> MERLVWDKLTLLGFLEKNHIPQKLYYNLSSQDKELSAEIQSNVTYYTLRDANNTLIQALIPISQDLQIHIYKKGEDYFLDFIPIIFTRKEKTLLLSLQTSPYQDIIKATNDPLLANQLMNAYKKSVPFKRLVKNDKIAIVYTRDYRVGQAFGQPTIKMAMVSSRSNQYYLFSHSNGHYYDSKAQEVAGFLLETPVKYTRISSPFSYGRFHPVLKVRRPHYGVDYAAKHGSLIHSASDGRVGFMGVKAGYGKVVEIHLNELRLVYAHMSAFANGLKKGSFVKKGQIIGRVGSTGLSTGPHLHFGVYKNSRPINPLGYIRTAKSKLHGKQREVFLEKAQRSKQKLEELLKTHSFEKNSFYLLEGFLEHHHHHH

Seven cell shape-determining genes (csd1, csd2, csd3/hdpA, ccmA, csd4, csd5 and csd6) have been identified in H. pylori. Among them, Csd3 (also known as HdpA) is a bifunctional enzyme. Its d,d-endopeptidase activity cleaves the d-Ala4-mDAP3 peptide bond between cross-linked muramyl tetrapeptides and pentapeptides.

Among these, only the N-terminally 41-residue truncated Csd3 (Csd3Δ41) comprised of residues 42–403 was expressed in soluble form, and it yielded two different forms (the orthorhombic form 1 and the hexagonal form 2) of well diffracting crystals. We have determined the structure of Csd3Δ41 using SAD data from a Pt-derivatized form 2 crystal. The form 2 crystal contains one monomer of Csd3Δ41 in the asymmetric unit. This model of Csd3Δ41 excludes six residues (Pro251–Arg256) in a disordered loop near the metal-binding site as well as four residues Gly333–Thr336 and two histidines at the end of the C-terminal affinity tag. In the form 1 crystal, the two monomers in the asymmetric unit bury a relatively large surface area of 1130 Å2 per monomer (6.0% of the monomer surface area), whereas the largest buried surface area in the form 2 crystal is 710 Å2 per monomer (3.8% of the monomer surface area). Loop I of Csd3 shows the most significant deviation among the homologues. In form 2 crystals, it is not involved in crystal packing and is disordered. Interestingly, the side chain of His339 of Csd3, the first histidine of the HxH motif, shows two different orientations. Its orientation in the form 2 crystals is similar to those in other homologous proteins. In both the form 1 and the form 2 crystals, domain 1 blocks the active-site cleft of the LytM domain, with the protruding helix α3 contributing to the Zn2+ coordination sphere.1-[(4-cyclohexylbutanoyl)(2-hydroxyethyl)amino]-1-deoxy-D-glucitol 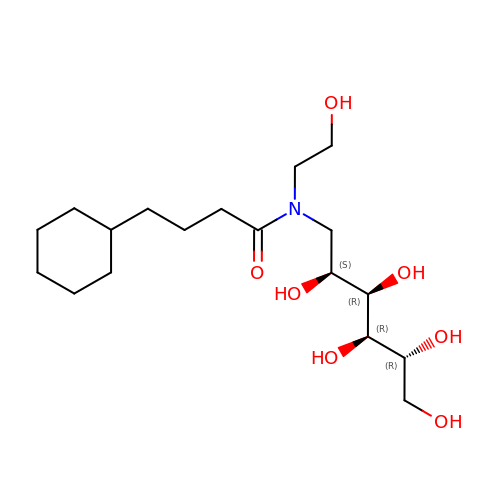| C18 H35 N O7 | XAMJEPWYNXYYBT-BURFUSLBSA-N>[4x]MKVVKEFSVCGGRLIKLSHNSNSTKTSMNV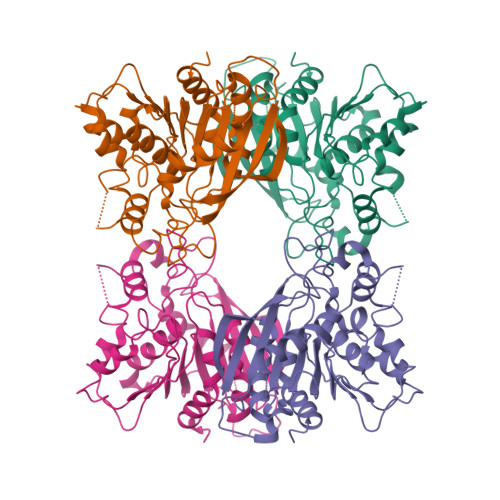NIYLPKHYYAQDFPRNKRIPTVFYLSGLTCTPDNASEKAFWQFQADKYGFAIVFPDTSPRGDEVANDPEGSWDFGQGAGFYLNATQEPYAQHYQMYDYIHKELPQTLDSHFNKNGDVKLDFLDNVAITGHSMGGYGAICGYLKGYSGKRYKSCSAFAPIVNPSNVPWGQKAFKGYLGEEKAQWEAYDPCLLIKNIRHVGDDRILIHVGDSDPFLEEHLKPELLLEAVKATSWQDYVEIKKVHGFDHSYYFVSTFVPEHAEFHARNLGLI(2S)-5-hydroxy-2-(4-hydroxyphenyl)-4-oxo-3,4-dihydro-2H-1-benzopyran-7-yl 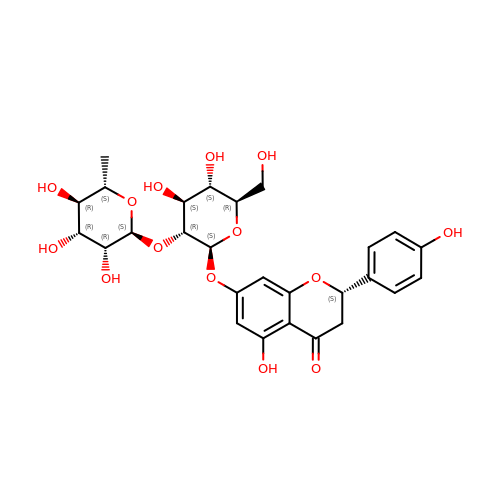2-O-(6-deoxy-alpha-L-mannopyranosyl)-beta-D-glucopyranoside | C27 H32 O14 | DFPMSGMNTNDNHN-ZPHOTFPESA-N>PPYTIVYFPVRGRCEAMRMLLADQGQSWKEEVVTIDTWMQGLLKPTCLYGQLPKFEDGDLTLYQSNAILRHLGRSLGLYGKNQREAAQMDMVNDGVEDLRGKYVTLIYTNYEN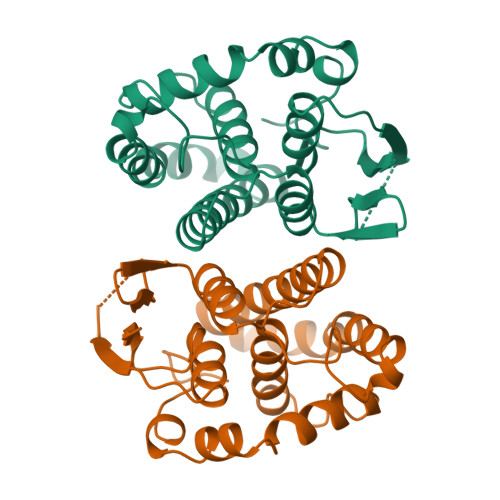GKNDYVKALPGHLKPFETLLSQNQGGKAFIVGDQISFADYNLLDLLLIHQVLAPGCLDNFPLLSAYVARLSARPKIKAFLSSPEHVNRPINGNGKQ[2x]> MEPVDPRLEPWKHPGSQPKTACTNCYCKKCC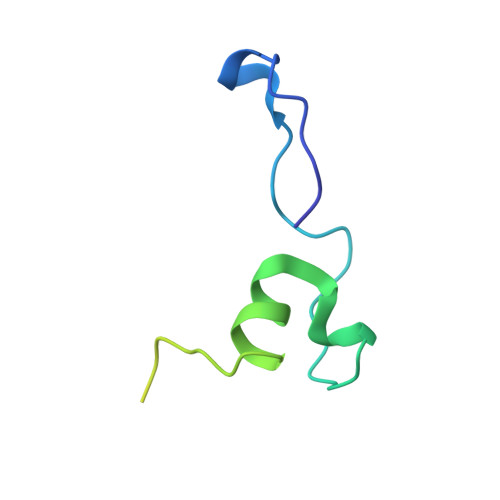FHCQVCFITKALGISYGRKKRRQRRRAHQNSQTHQASLSKQPTSQSRGDPTGPKE The lasso peptide MS-271 is a ribosomally synthesized and post-translationally modified peptide (RiPP) consisting of 21 amino acids with D-tryptophan at the C-terminus, and is derived from the precursor peptide MslA. MslH, encoded in the MS-271 biosynthetic gene cluster (msl), catalyzes the epimerization at the Cα center of the MslA C-terminal Trp21, leading to epi-MslA. Herein, based on X-ray crystallographic studies in association with MslA core peptide analogues, we show that MslH is a metallo-dependent peptide epimerase with a calcineurin-like fold. The crystal structure analysis, followed by site-directed mutagenesis, docking simulation, and ICP-MS studies demonstrate that MslH employs acid/base chemistry to facilitate the reversible epimerization of the C-terminal Trp21 of MslA, by utilizing two pairs of His/Asp catalytic residues that are electrostatically tethered to a six-coordination motif with a Ca(II) ion via water molecules.

Hence, recombinant N-terminally His6-tagged MslAΔTrp21, which lacked the C-terminal Trp21, and MslA Trp21G variants, with an achiral glycine instead of Trp21, were prepared by co-expression with MslB1 in E. coli. As a result, the X-ray crystal structures of the MslH:MslAΔTrp21 and MslH:MslA Trp21G complexes at 2.29 Å and 2.12 Å resolutions, respectively, with one monomer in the asymmetric unit, which are the same as the MslH:apo structure, were successfully obtained. The electron density of MslAΔTrp21 in the MslH:MslAΔTrp21 crystal structure allowed us to locate a cyclic peptide molecule (cMslA Gly12-Phe20), consisting of the Gly12-Phe20 part on the C-terminal side of MslAΔTrp21 with a disulfide bond between Cys13 and Cys19, in the large cleft conformed by two monomers. However, no electron density corresponding to either the MslA leader peptide or MslB1 was identified in the MslH:MslAΔTrp21 crystal structure. The cMslA Gly12-Phe20 of MslAΔTrp21 molecule is accommodated in the cleft with various interactions, such as a σ–π interaction between Phe228 of monomer A and Tyr15 in cMslA Gly12-Phe20 (3.8 Å), hydrophobic interactions between α6’ of monomer B and MslA Ala16-Val18, and polar interactions between Gly60 (3.4 Å)/His295 (2.7 Å) in MslH and the carboxyl group of the C-terminal MslA Phe20 of MslAΔTrp21. In addition, an architecture that would construct a six-coordination motif, consisting of four amino acid residues Glu44, Asn87, His259, and His261 and two water molecules (w1 and w2), was detected around the C-terminal carboxyl group of MslA Phe20 in the MslH:MslAΔTrp21 crystal structure. In the six-coordination, the w2 water molecule hydrogen-bonds with the side-chain of Asp11 and is further held in the structure by the steric contraction of the His295 side-chain, which forms a hydrogen-bond with Asp11. The in vitro enzymatic reaction indicated that the catalytic activity was maintained in MslH expressed in M9 medium, as in the case of the recombinant MslH expressed in Luria-Bertani (LB) medium.

> MTRLTVALSGDCMVTRGGLITSDPAAERLRDLLRGTDFAVTNLEVVPSDGRGHPVHNAVGGGCLIADSAVLDEVTAAGFSVLGCANNHAMDLGTEGVLGTMDLLRARGIPYAGIGADLTGARRPVYADRPGGSLALLSCTATFLPGQEAADPSPELPGRPGLNPLRHTATMQVTADQMDVLRTIDAETGLRARRAEARALLGVDPALLGPDRLALFGTRFRTADAPGFTTECDPRDLDEIARWVGEARLRADLVVVSVHSHEPGPTPETPGEFLRVFAHRMIDEGAHAVVGHGPHFLRGVELYRNKPIFYSLGNIVSQIELTDRVSAEDYAKVTAERPLTPGRYYDRLSGHGTRLFAPHRRYWQSLVPVLTFEDGTLTAARLHPVDLGFGRPVHRRGRPRLADRAEAEKTLTDVAQLSQPYGTAIEVMDDGTGELALDVA;> CLGVGSCNDFAGCGYAIVCF(2S)-3-cyclohexyl-2-(6-fluoro-4-oxoquinazolin-3(4H)-yl)-N-(1,3-thiazol-2-yl)propanamide | C20 H21 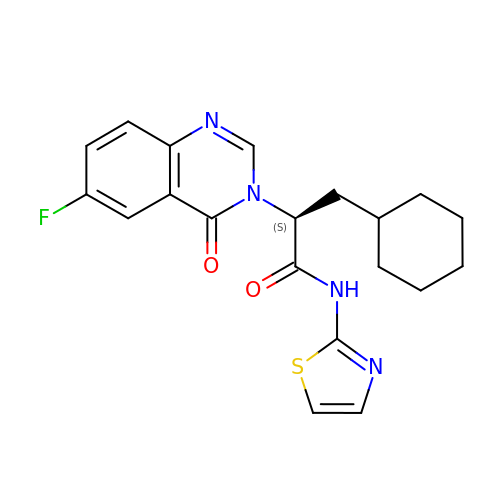F N4 O2 S | HETBALZVBPDEQB-KRWDZBQOSA-N1-(4-{4-morpholin-4-yl-1-[1-(pyridin-3-ylcarbonyl)piperidin-4-yl]-1H-pyrazolo[3,4-d]pyrimidin-6-yl}phenyl)-3-pyridin-4-ylurea 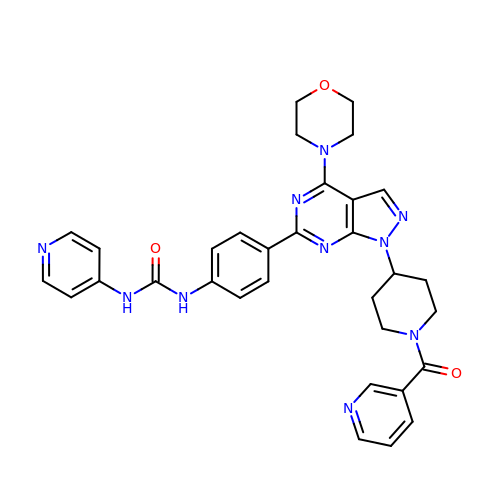| C32 H32 N10 O3 | HLHOHTNONYACFD-UHFFFAOYSA-N> SNAMANVKLLLPYILKWE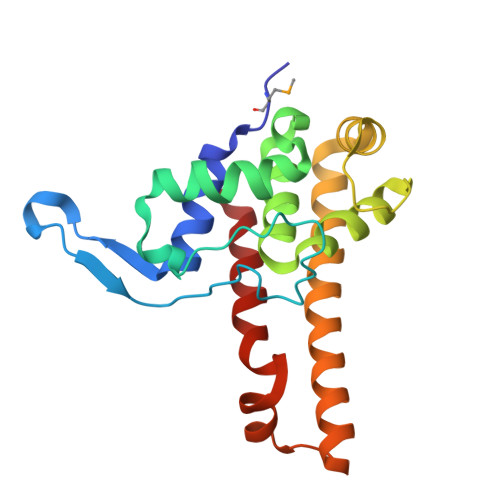GGFVHDPADAGGATNKGVTIATWKRVGYDKDGDGDIDVEDLKLLTDDDVLNRVLKPFYWDRWKADLIESQKVANILVDWVWGSGKYGIVIPQRILGVQADGIVGNKTLQAVNSADPDELFESIFDARREFLEDITARSIKKYEDSIGRKATERELLRHTNKRFLRGWLNRLEDIRKL> SPLKLQSRKLRYANDVQ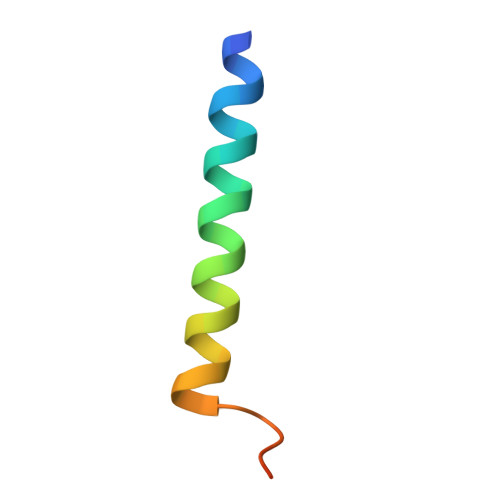DLLDDVENSPVVATKRQNV> MSLERRTLIMEVLFEAKVGDITLKLAQGDITQYPAKAIVNAANKRLEHGGGVAYAIAKACAGDAGLYTEISKKAMREQFGRDYIDHGEVVVTPAMNLEERGIKYVFHTVGPICSGMWSEELKEKLYKAFLGPLEKAEEMGVESIAFPAVSAGIYGCDLEKVVETFLEAVKNFKGSAVKEVALVIYD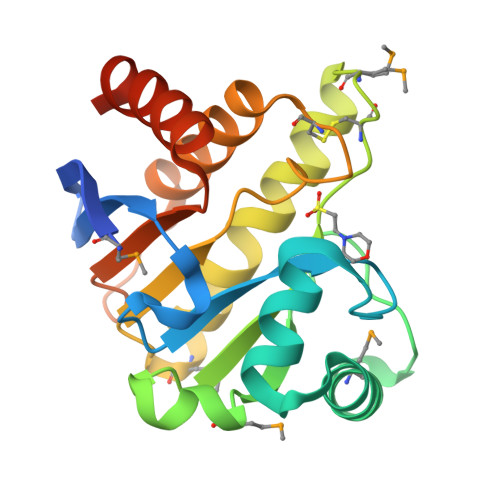RKSAEVALKVFERSLEGGSHHHHHH>[4x]GSFIDIEFPEWFHEGLSRHQAENLLMGKDIGFFI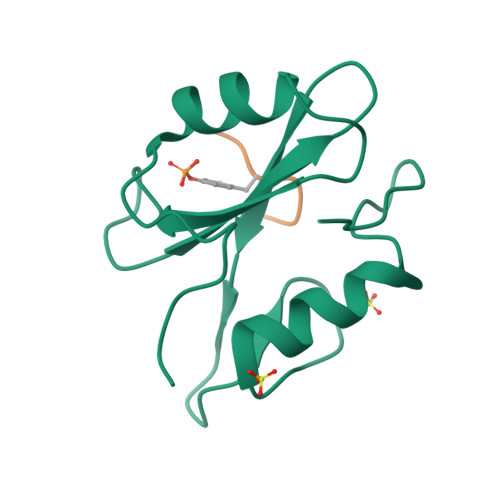IRASQSSPGDFSISVRHEDDVQHFKVMRDTKGNYFLWTEKFPSLNKLVDYYRTTSISKQKQVFLRD;>[4x]XPDYENL Among diverse BMCs, carboxysomes are specific CO2-fixing BMCs found in all cyanobacteria and many proteobacteria. The carboxysome uses a polyhedral protein shell to encapsulate the key CO2 fixation enzymes, ribulose-1,5-bisphosphate carboxylase/oxygenase (Rubisco) and carbonic anhydrase (CA). Carboxysome shells are typically composed of three groups of structural components that form hexamers, pentamers, and trimers. Here, we generated recombinant α-carboxysome shells of Halothiobacillus neapolitanus by expressing all the shell proteins (involving three CsoS1 hexameric proteins and two CsoS4 pentameric proteins), together with the C-terminal domain of CsoS2 (CsoS2-C) that mediates shell assembly.

The cryo-EM structures of T = 9, T = 9 Q = 12, T = 13, T = 16, and T = 19 shell assemblies were determined at 2.3-, 2.99-, 2.93-, 2.75-, and 3.04-Å resolution, respectively. The resulting shell structures show various sizes, with a maximal size of 54 nm, representing the largest synthetic icosahedral BMC shells to date that are suitable for in-depth structural analysis. The T = 9 shell has a minimum of four different interfaces, whereas the T = 19 shell has a maximum of 10 different interfaces. Notably, structural analysis of the large T = 19 shell revealed the highest number of CsoS2-C fragments and additional binding details. The five fragments cover a substantial portion of entire CsoS2-C (Ser604-Gly869). F3 and F4 belong to the same region of CsoS2-C (Ile702-Arg735). Closer inspection revealed that F3 has a sequence overlap with F4, although their conformations differ. Nevertheless, our results indicate that CsoS2-C adopts at least two distinct conformations for interacting with the shell. Intriguingly, the smaller T = 9 shells involved only one conformation of CsoS2-C, whereas the second conformation of CsoS2 appeared in the larger T = 13, T = 16, and T = 19 shells.

>[18x]MADVTGIALGMIETRGLVPAIEAADAMTKAAEVRLVGRQFVGGGYVTVLVRGETGAVNAAVRAGADACERVGDGLVAAHIIARVHSEVENILPKAPQA;> MKIMQVEKTLVSTNRIADMGHKPLLVVWEKPGAPRQVAVDAIGCIPGDWVLCVGSSAAREAAGSKSYPSDLTIIGIIDQWNGE;>MPFCTSTPEPEAQSTEQSLTCEGQIISGTSVDASDLVTGNEIGEQQLISGDAYVGAQQTGCLPTSPRFNQTGNVQSMGFKNTNQPEQNFAPGEVMPTDFSIQTPARSAQNRITGNDIAPSGRITGPGMLATGLITGTPEFRHAARELVGSPQPMAMAMANRNKAAQAPVVQPEVVATQEKPELVCAPRSDQMDRVSGEGKERCHITGDDWSVNKHITGTAGQWASGRNPSMRGNARVVETSAFANRNVPKPEKPGSKITGSSGNDTQGSLITYSGGARG[2x]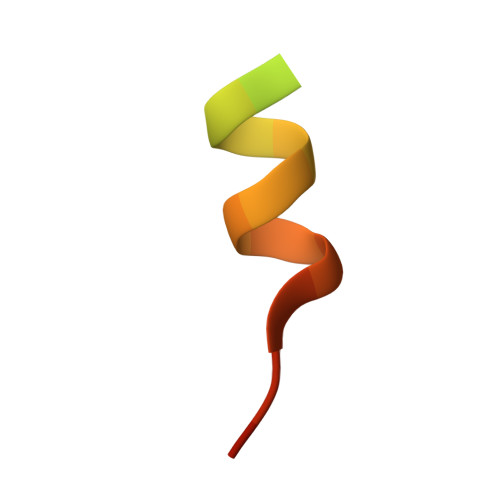> LERNNIKQAANNSLLLHLLKSQTIP> TGSSLP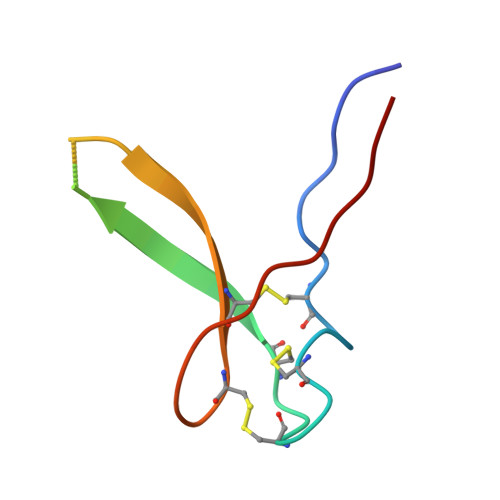DCSYACGACSPCKRVMISFECSVAESCSVIYRCTCRGRYYHVPSRA> GSPGIPPAPGDFSGEGSQGLPDPSPEPKQLPELIRMKRDGGRLSEADIRGFVAAVVNGSAQG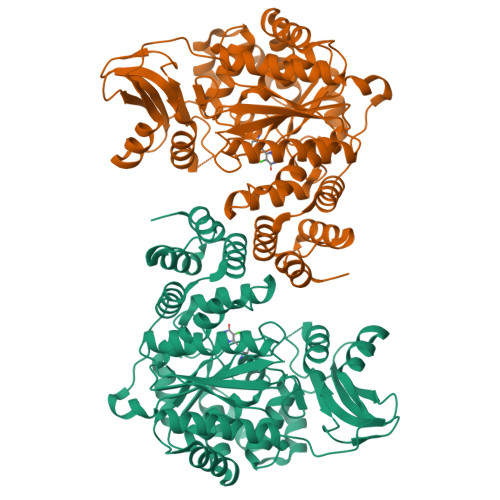AQIGAMLMAIRLRGMDLEETSVLTQALAQSGQQLEWPEAWRQQLVDKHSTGGVGDKVSLVLAPALAACGCKVPMISGRGLGHTGGTLDKLESIPGFNVIQSPEQMQVLLDQAGCCIVGQSEQLVPADGILYAARDVTATVDSLPLITASILSKKLVEGLSALVVDVKFGGAAVFPNQEQARELAKTLVGVGASLGLRVAAALTAMDKPLGRCVGHALEVEEALLCMDGAGPPDLRDLVTTLGGALLWLSGHAGTQAQGAARVAAALDDGSALGRFERMLAAQGVDPGLARALCSGSPAERRQLLPRAREQEELLAPADGTVELVRALPLALVLHELGAGRAGEPLRLGVGAELLVDVGQRLRRGTPWLRVHRDGPALSGPQSRALQEALVLSDRAPFAAPLPFAELVLPPQQ2,6-dimethoxyphenol | C8 H10 O3 | 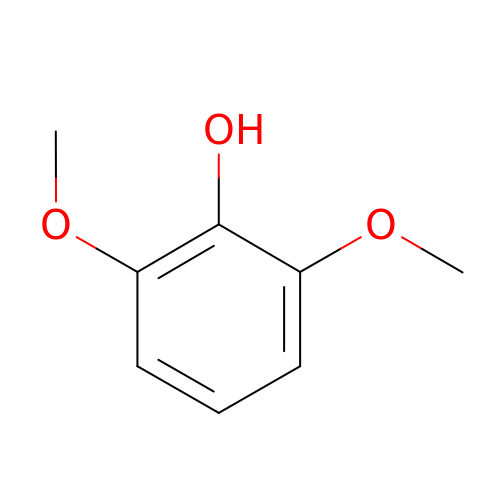KLIDCXVFHGNTTM-UHFFFAOYSA-N(R)-2-(FORMYLOXY)-3-(PHOSPHONOOXY)PROPYL PENTANOATE 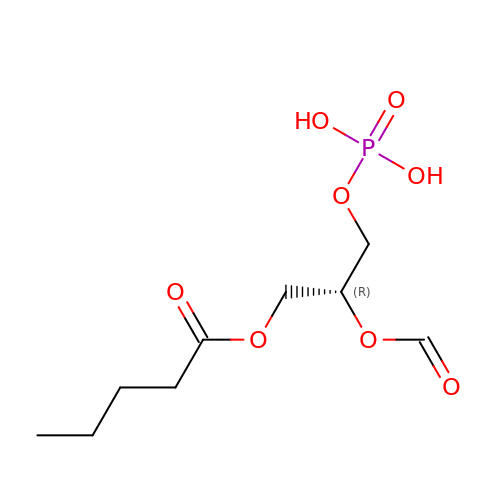| C9 H17 O8 P | JDTMNMAQWVSSOO-MRVPVSSYSA-N7-{[3-({[(pyridin-2-yl)methyl]amino}methyl)phenyl]methoxy}-5,8-dihydroquinolin-2-amine | C23 H24 N4 O | 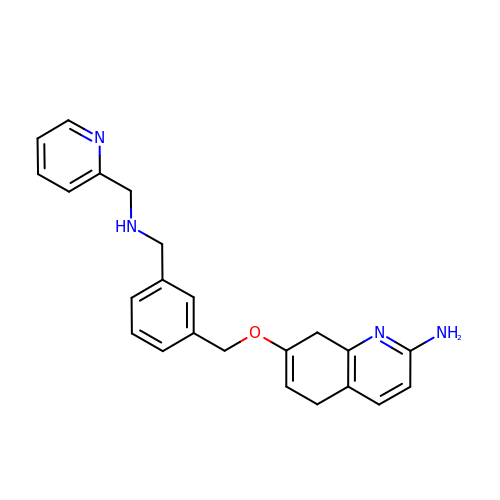KJHXGBWLZFPKIP-UHFFFAOYSA-N> SMEPYEKEVAEYNKHKNENSYVNEAISKNLVFDQSVVTKDTKISSIKGGKFIKATDFNKVNAGDSKDIFTKLRKDMGGKATGNFQNSFVKEANLGSNGGYAVLLEKNKPVTVTYTGLNASYLGRKITKAEFVYELQSSPSQSG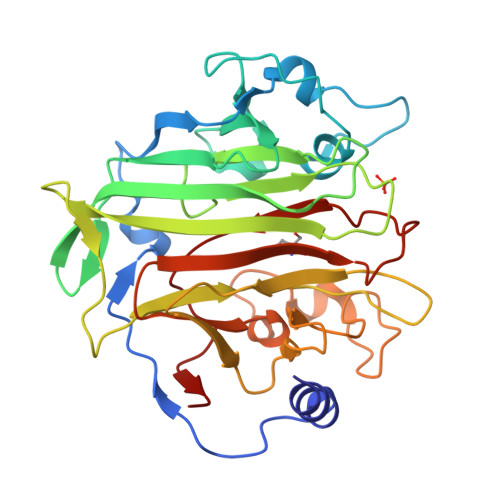TLNAVFSNDPIITAFIGTNRVNGKDVKTRLTIKFFDASGKEVLPDKDSPFAYALSSLNSSLTNKGGHAEFVSDFGANNAFKYINGSYVKKQADGKFYSPEDIDYGTGPSGLKNSDWDAVGHKNAYFGSGVGLANGRISFSFGMTTKGKSNVPVSSAQWFAFSTNLNAQSVKP3-[(2R,3aR,5R,6R,6aR)-5-({[(S)-{[(S)-{[(2R,3S,4R,5R)-5-(6-amino-9H-purin-9-yl)-3,4-dihydroxytetrahydrofuran-2-yl]methoxy}(hydroxy)phosphoryl]oxy}(hydroxy)phosphoryl]oxy}methyl)-2,6-dihydroxytetrahydrofuro[2,3-d][1,3]oxathiol-2-yl]propanoic acid 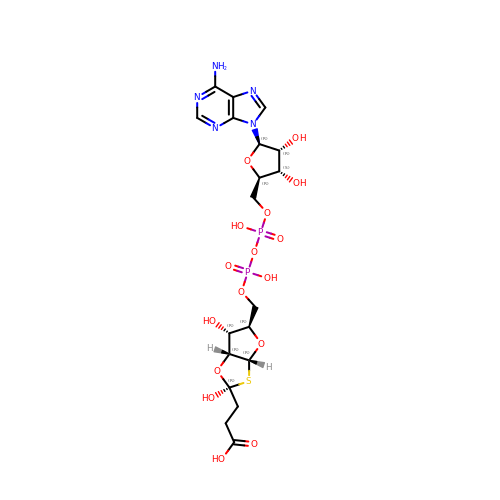| C19 H27 N5 O16 P2 S | DLPJYEOHCQEPAR-IOFPOCHNSA-N> GVPETRPNHTIYINNLNEKIKKDELKKSLYAIFSQFGQILDILVSRSLKMRGQAFVIFKEVSSATNALRSMQGFPFYDKPMRIQYAKTDSDIIAKMKGTFVERDRKREKRGSGSGSGSGSGSGAETREERMERKRREKIERRQQEVETELKMWDPHNDPNAQGDAFKTLFVARVNYDTTESK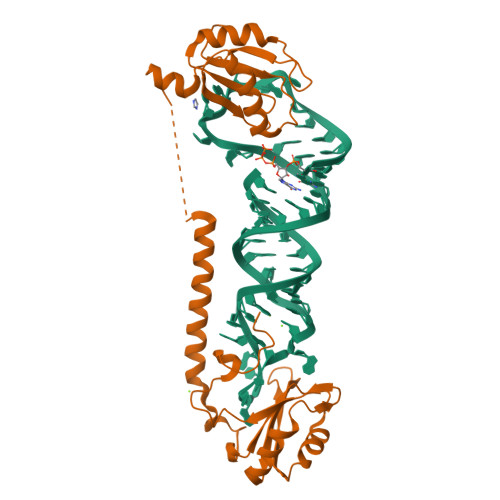LRREFEVYGPIKRIHMVYSKRSGKPRGYAFIEYEHERDMHSAYKHADGKKIDGRRVLVDVERGRTVKGWRPRRLGGGLGGTRRGGADVNIRHSGRDD3,5-dideoxy-5-[(methoxycarbonyl)amino]-D-glycero-alpha-D-galacto-non-2-ulopyranosonic acid | C11 H19 N O10 | 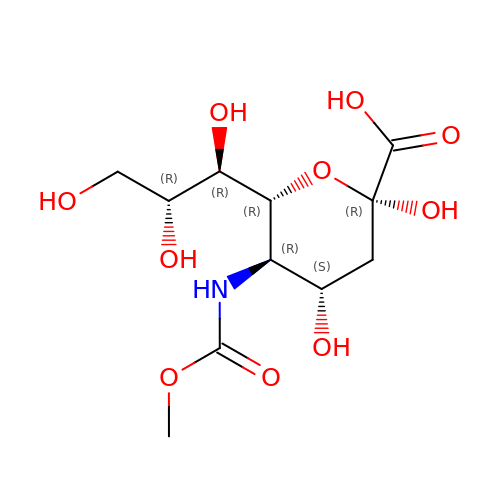CBSUGMQOJBEHIX-HSASFHKOSA-N>[4x]MKKVEAIIRPF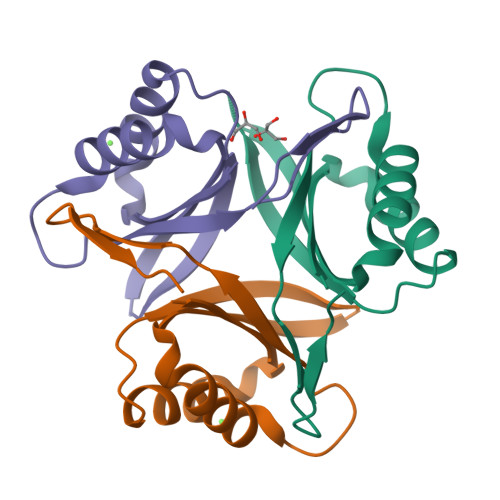KLDEVKIALVNAGIVGMTVSEVRGFGRQKGQTERYRGSEYTVEFLQKLKIEIVVDEGQVDMVVDKLVSAARTGEIGDGKIFISPVDSVVRIRTGEKDTEAI> DG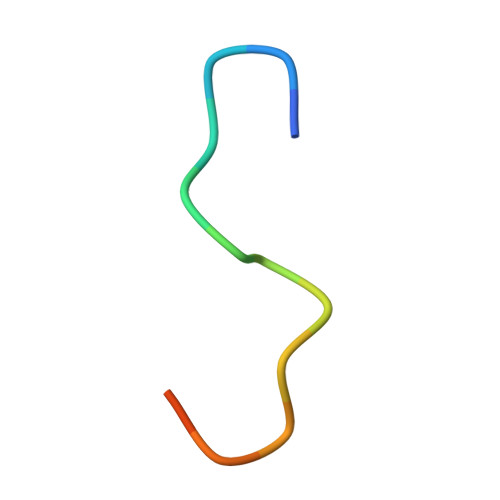VFTTPCDPEYAGG PGAM5 is a mitochondrial membrane protein that functions as an atypical Ser/Thr phosphatase and is a regulator of oxidative stress response, necroptosis, and autophagy. Phosphoglycerate mutase family member 5 (PGAM5) is a mitochondrial membrane protein that belongs to the phosphoglycerate mutase (PGAM) branch of the histidine acid phosphatase superfamily, known also as two-histidine phosphatase (2H-phosphatase). Despite harboring a canonical RHGE catalytic motif, PGAM5 lacks a typical phosphotransferase and/or phosphohydrolase activity for small metabolites, and displays instead a phosphatase function specific for Ser/Thr and, potentially, histidine residues (Takeda et al., 2009, Panda et al., 2016). Overall, the catalytic domain of PGAM5 adopted a classical phosphoglycerate mutase-like fold with the canonical three-layer sandwich topology, which featured a six-stranded β sheet flanked on both sides by α helices with the first four parallel strands arranged in an alternated β/α manner.

Among a series of truncated proteins, the ΔN90-PGAM5 construct harboring the catalytic domain readily crystallized, enabling high-resolution structure determination to 1.70 Å. The last two strands formed an antiparallel arrangement, projecting the C-terminal tail in proximity to the active site situated on top of the β-sheet core. The two molecules of PGAM5 in the crystallographic asymmetric unit demonstrated a dimeric arrangement. Both subunits associated by aligning the β-sheet cores along the non-crystallographic two-fold symmetry with their active sites located at distal sites. Intermolecular interactions were exclusively constrained to the C-terminal portions, where the α4-β5 loop, β6 strand, and C-terminal tail from one molecule packed against the corresponding region in the other protomer. Unlike the α4-β5 loop and β6 strand, the contribution of the C-terminal tails to dimeric intersubunit contacts was limited to only one hydrogen bond between the β6 D277 and the tail residue G279, prompting us to investigate the role of this region regarding the stability of the dimer. Consistently, the deletion of the C-terminal tail (ΔC-tail) almost completely abolished the association of this construct with full-length protein, an ability that was highly maintained in the other truncated variants retaining the C-terminal tail. These results therefore suggested that the C-terminal tail played an important stabilizing role in the dimeric assembly, which was also supported by the dissociation constant (KD) of ∼0.48 μM determined for the construct “d” (residues 90–289) by AUC equilibrium sedimentation experiments. As expected, the catalytic domain alone (ΔN90) lacked an ability to form large assemblies, and existed as a dimer in solution even at high protein concentration.

>[2x]SMDHYKAKATRHIFLIRHSQYHVDGSLEKDRTLTPLGREQAELTGLRLASLGLKFNKIVHSSMTRAIETTDIISRHLPGVCKVSTDLLREGAPIEPDPPVSHWKPEAVQYYEDGARIEAAFRNYIHRADARQEEDSYEIFICHANVIRYIVCRALQFPPEGWLRLSLNNGSITHLVIRPNGRVALRTLGDTGFMPPDKITRS> GPGSEFGNSARIP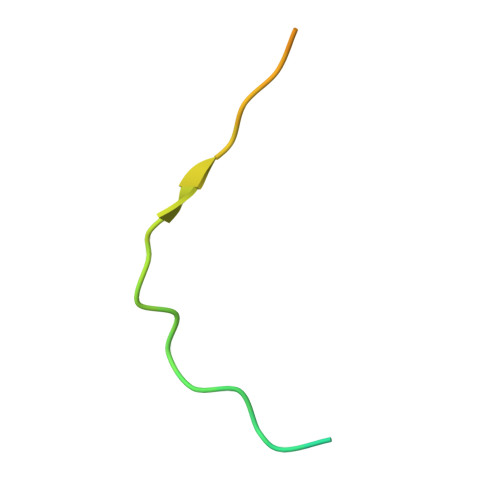CPKTRLARVSVLDLKKIEEQPDSSSG> SNAMTNRYTTLFANLEKRNEGAFIPFVTIGDPNKALSFEIIDTLVSSGADALELGIPFSDPLADGPTIQEANIRALESGITPKDCFDILTKIRAKYPHIPIGLLLYANLVYANGIENFYQKCLDAGVDSILIADVPAHESKEFRDIAKKVGIAQIFIAPPDASESTLKQISELGSGYTYLLSRVGVTGTETAANMPVEDVLTKLREYNAPKPVLGFGISKPEQVQQAIKAGAAGAISGSATVKIIQNNISNKQKMLNELTYFVKEMKAATLN;> MSKLNAYFGEYGGQFVPQILVPALDQLEQEFIKAQADESFKQEFKELLQEYAGRPTALTKTRNIVKNTRTKLYLKREDLLHGGAHKTNQVLGQALLAKRMGKKEIIAETGAGQHGVATALACALLDLKCRVYMGAKDVERQSPNVFRMKLMGAEVIPVHSGSATLKDACNEALRDWSANYSKAHYLLGTAAGPHPFPTIVREFQRMIGEETKQQMLAKEGRLPDAVIACVGGGSNAIGMFADFIDEKNVKLIGVEPAGKGIETGEHGAPLKHGKTGIFFGMKAPLMQNSDGQIEESYSISAGLDFPSVGPQHAHLLAIGRAKYASATDDEALDAFKLLCKKEGIIPALESSHALAHALKLAYEDPNKEQLLVVNLSGRGDKDIFTVHDILKEKGEI

Tryptophan synthase (TrpAB) is a pyridoxal 5′-phosphate (PLP)-dependent enzyme that participates in the final two steps of tryptophan synthesis in plants, fungi and bacteria. The enzyme consists of two protein chains, α (TrpA) and β (TrpB), that operate as a linear αββα heterotetrameric complex containing two functional TrpAB units. In bacteria, TrpA and TrpB are encoded by usually adjacent trpA and trpB genes that belong to the highly regulated tryptophan-biosynthesis operon. The TrpA subunit converts indole-3-glycerol phosphate (IGP) into glyceraldehyde 3-phosphate (G3P) and indole (IND).

Similarly, in TrpB (amino-acid residues 4–407) the N-terminal SNA sequence and the C-terminal end (residues 403–407) are not present in the respective chains B and D. The other ortholog, FtTrpAB, crystallized in space group C2221 and the asymmetric unit contains only one αβ module. This structure was solved by experimental SAD phasing and was refined to 2.80 Å resolution. In FtTrpAB, TrpA (chain A; residues 1–269) lacks the N-terminal SNA sequence and residues 183–191, while in TrpB (chain B; residues 1–396) the C-terminal residue is not present. The level of pairwise sequence identity between the TrpBs from these organisms ranges from 51% to 59%, with the exception of the FtTrpB/StTrpB pair, which show 81% conserved residues. The enzyme from F. tularensis, which is the most closely related to StTrpAB, shows even better agreement, with an r.m.s.d. of 0.8 Å for corresponding StTrpA Cα atoms. The structures of the FtTrpAB and SpTrpAB αββα heterotetramers provide a new set of high-quality models and enable comparison of the intermolecular tunnel connecting the TrpA and TrpB catalytic pockets. In contrast to the active sites, the composition of the tunnel, which is mostly encompassed by TrpB, varies between the orthologs, although generally SpTrpAB shares some features with MtTrpAB while FtTrpAB is similar to StTrpAB. The MVC is indirectly connected to the βH6 element of the COMM domain and to TrpA via either a histidine (βHis285Sp and βHis294Mt) or a phenylalanine (βPhe279Ft, βPhe280St), switching between hydrophobic Phe–Phe contacts (FtTrpB and StTrpB) and the well defined His–Tyr hydrogen bond seen in MtTrpB and most likely to be present in the activated form of SpTrpB. While no monovalent cations have been modeled in the current structures, by analogy to the data collected from the MtTrpAB and StTrpAB systems the MVC must be created by βTyr311Sp, βGly313Sp, βAla273Sp, βGly237Sp and βThr275Sp in SpTrpAB and βPhe305Ft, βSer307Ft, βGly267Ft, βGly231Ft in FtTrpAB, with βPro269Ft replacing the threonine residue. The specific activity order is as follows: FtTrpAB >> MtTrpAB, SpTrpAB >> LpPhTrpAB.> MTNLAPANSEKIRVDIWSDIACPWCYIGKRRFESALGQFPQRDQVEVVWHSFELDPSARPLNPIAMRDGLAMKYSISPAQAQGSLDHMTQTAAQEGLEYHFDRVKLANTFLAHQLIHYAAEQGQGDAMKERLLRAYMSEGQNVNDLDTLQKLAAEVGLDAGAARAALEAGTYAQAVRYD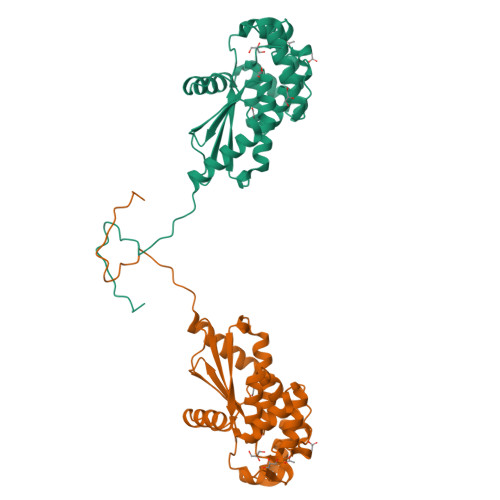EAQAQQLGITGVPFFVLGGKYGVSGAQAPETLLGALSQVWAEQHPAPLTMLGQDAPAEGSEDGQCAVPQRPNNLEHHHHHH>[2x]GKSDKIIPIAENKEAKAKYDILETYEA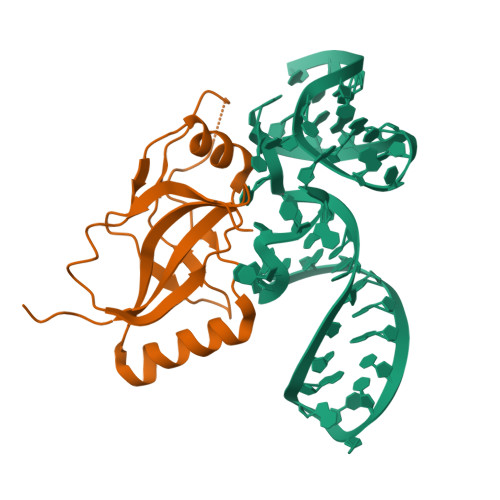GIVLKGSEVKSLREKGTVSFKDSFVRIENGEAWLYNLYIAPYKHATIENHDPLRKRKLLLHKREIMRLYGKVQEKGYTIIPLKLYWKNNKVKVLIALAKGKKLYDRRRELKEKAMKRELEREFKGKIHL>METSKEKTITSPGPYIVRLLNSSLNGCEFPLLTGRTLFVVGQSDALTASGQLPDIPADSFFIPLDHGGVNFEIQVDTDATEIILHELKEGNSESRSVQLNTPIQVGELLILIRPESEPWVPEQPEKLETSAKKNEPRFKNGIVAALAGFFILGIGTVGTLWILNSPQRQAAELDSLLGQEKERFQVLPGRDKMLYVAAQNERDTLWARQVLARGDYDKNARVINENEENKRISIWLDTYYPQLAYYRIHFDEPRKPVFWLSRQRNTMSKKELEVLSQKLRALMPYADSVNITLMDDVTAAGQAEAGLKQQALPYSRRNHKGGVTFVIQGALDDVEILRARQFVDSYYRTWGGRYVQFAIELKDDWLKGRSFQYGAEGYIKMSPGHWYFPSPL[24x];>MIRRYLYTFLLVMTLAGCKDKDLLKGLDQEQANEVIAVLQMHNIEANKIDSGKLGYSITVAEPDFTAAVYWIKTYQLPPRPRVEIAQMFPADSLVSSPRAEKARLYSAIEQRLEQSLQTMEGVLSARVHISYDIDAGENGRPPKPVHLSALAVYERGSPLA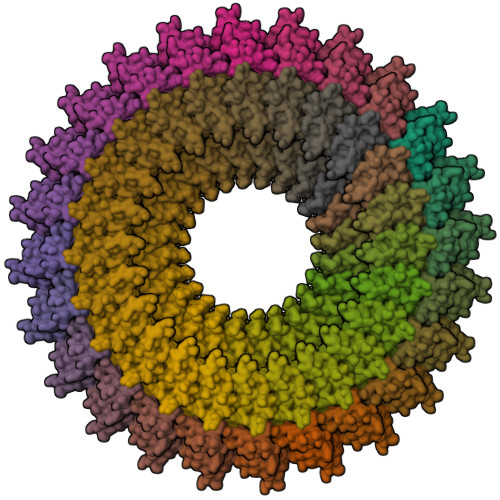HQISDIKRFLKNSFADVDYDNISVVLSERSDAQLQAPGTPVKRNSFATSWIVLIILLSVMSAGFGVWYYKNHYARNKKGITADDKAKSSNE[24x]> CEKQVQEVGLDGTETYLQPLSMSQNL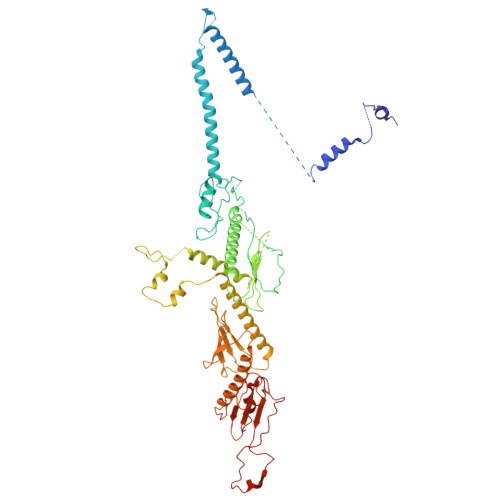ARLAQRIDFSQGSGSEEEEAAGPDGDAPDWGGAGADQDDEEGLVKFQPSLWPWDSVRNNLRSALTEMCVLYDVLSIVRDKKFMTLDPVSQDALPPKQSPQTLQLISKKKSLAGAAQILLKGAERLTKSVAENQENKLQRDFNSELLRLRQHWKLRKVGDKILGDLSYRSAGSLFPHHGTFEVIKNTDIDLDKKIPEDYCPLDVQIPSDLEGSAYIKVSIQKQAPDIGDLGTVNLFKRPLPKSKPGSPHWQTKLEAAQNVLLCKEIFAQLSREAVQIKSQIPHIVVKNQIISQPFPSLQLSISLCHSSDDKKSQKCAAEKPGQEDHLYVLEHNLHLLIREFHKQTLSSIVMPHPASAPFGHKRMRLSGPQAFDKNEINSIQSTEGLLEKIIKQAKHIFLRSRTAATIDSLASRIEDPQIQAHWSNINDVYESSVKVLITSQGYEQICKSIQLQLNIGVEQVRVVHRDGRVIMLSHQEQELQDFLLSQMSQHQVHAVQQLAKVMGWQVLSFSNHVGLGPIESIGNASAITVASPSGDYAISVRNGPESGSKIMVQFPRNQCKDLPKSDVLQDSKWSHLRGPFKEVQWNKMEGRNFVYKMELLMSALS> MSEY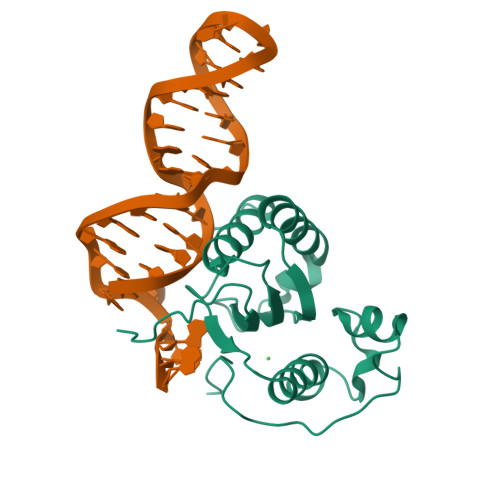RRYYIKGGTWFFTVNLRNRRSQLLTTQYQMLRHAIIKVKRDRPFEINAWVVLPEHMHCIWTLPEGDDDFSSRWREIKKQFTHACGLKNIWQPRFWEHAIRNTKDYRHHVDYIYINPVKHGWVKQVSDWPFSTFHRDVARGLYPIDWAGDVTDFSAGERIIS>[4x]MHHHHHHHKPEDFRASTQRPFTGEEYLKSLQDGREIYIYGERVKDVTTHPAFRNAAASVAQLYDALHKPEMQDSLCWNTDTGSGGYTHKFFRVAKSADDLRQQRDAIAEWSRLSYGWMGRTPDYKAAFGCALGANPGFYGQFEQNARNWYTRIQETGLYFNHAIVNPPIDRHLPTDKVKDVYIKLEKETDAGIIVSGAKVVATNSALTHYNMIGFGSAQVMGENPDFALMFVAPMDADGVKLISRASYEMVAGATGSPYDYPLSSRFDENDAILVMDNVLIPWENVLIYRDFDRCRRWTMEGGFARMYPLQACVRLAVKLDFITALLKKSLECTGTLEFRGVQADLGEVVAWRNTFWALSDSMCSEATPWVNGAYLPDHAALQTYRVLAPMAYAKIKNIIERNVTSGLIYLPSSARDLNNPQIDQYLAKYVRGSNGMDHVQRIKILKLMWDAIGSEFGGRHELYEINYSGSQDEIRLQCLRQAQNSGNMD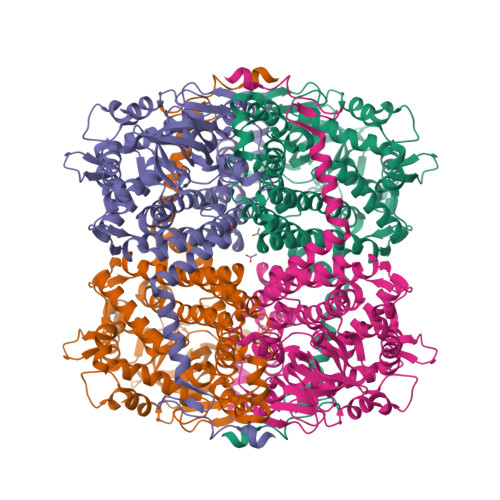KMMAMVDRCLSEYDQDGWTVPHLHNNDDINMLDKLLK>[2x]STAGKVIKCKAAVLWEEKKPFSIEEVEVAPPKAHEVRIKMVATGICRSDDHVVSGTLVTPLPVIAGHEAAGIVESIGEGVTTVRPGDKVIPLFTPQCGKCRVCKHPEGNFCLKNDLSMPRGTMQDGTSRFTCRGKPIHH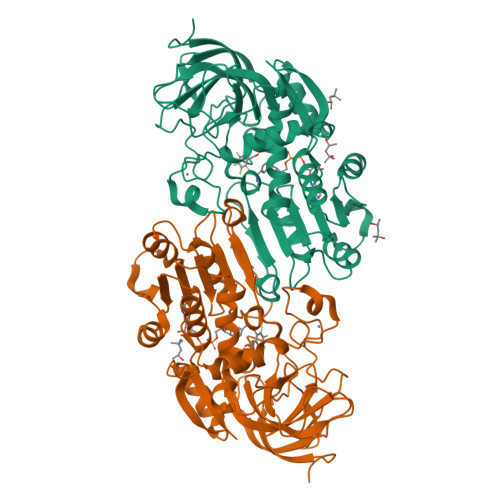FLGTSTFSQYTVVDEISVAKIDAASPLEKVCLIGCGFSTGYGSAVKVAKVTQGSTCAVFGLGGVGLSVIMGCKAAGAARIIGVDINKDKFAKAKEVGATECVNPQDYKKPIQEVLTEMSNGGVDFSFEVIGRLDTMVTALSCCQEAYGVSVIVGVPPDSQNLSMNPMLLLSGRTWKGAIFGGLKSKDSVPKLVADFMAKKFALDPLITHVLPFEKINEGFDLLRSGESIRTILTF>GAMGGSWEIDPKDLTFLKELGTGQFGVVKYGKWRGQYDVAIKMIKEGSMSEDEFIEEAKVMMNLSHEKLV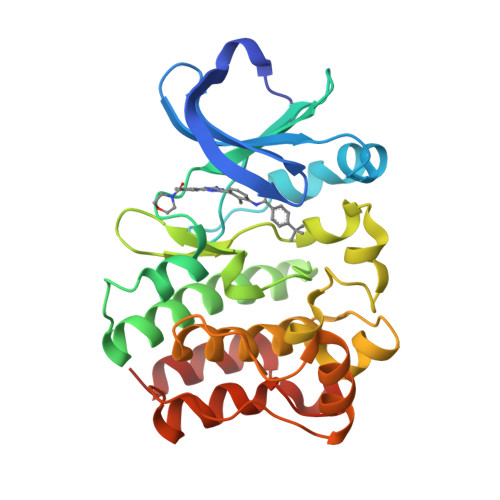QLYGVCTKQRPIFIITEYMANGCLLNYLREMRHRFQTQQLLEMCKDVCEAMEYLESKQFLHRDLAARNCLVNDQGVVKVSDFGLSRYVLDDEYTSSVGSKFPVRWSPPEVLMYSKFSSKSDIWAFGVLMWEIYSLGKMPYERFTNSETAEHIAQGLRLYRPHLASEKVYTIMYSCWHEKADERPTFKILLSNILDVMD[6x]> GSNEVNLLDSRTVMGDLGWIAFPKNGWEEIGEVDENYAPIHTYQVCKVMEQNQNNWLLTSWISNEGASRIFIELKFTLRDCNSLPGGLGTCKETFNMYYFESDDQNGRNIKENQYIKIDTIAADESFTELDLGDRVMKLN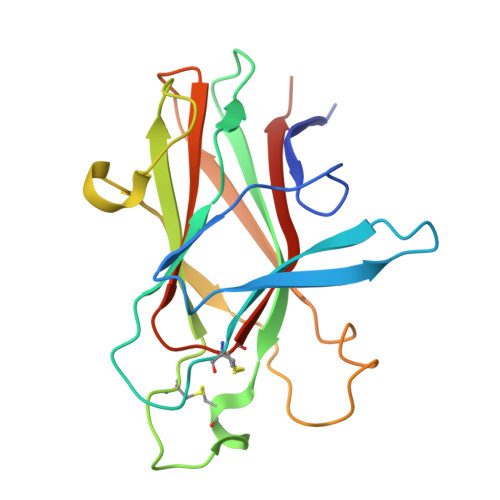TEVRDVGPLSKKGFYLAFQDVGACIALVSVRVYYKEAPS(7R)-2-[(3,5-difluoro-4-hydroxyphenyl)amino]-7,8-dimethyl-5-(prop-2-yn-1-yl)-7,8-dihydropteridin-6(5H)-one 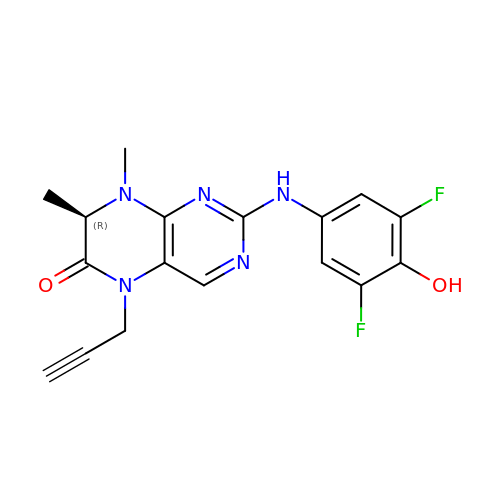| C17 H15 F2 N5 O2 | IIBALDWMKAODIG-SECBINFHSA-N> SQANLMRLKSDLFNRSPMYPGPTKDDPLTVTLGFTLQDIVKVDSSTNEVDLVYYEQQRW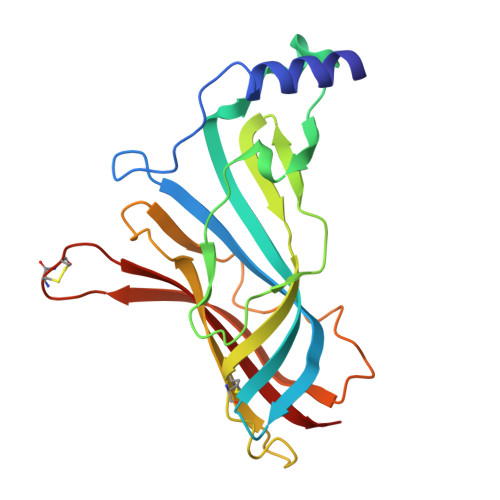KLNSLMWDPNEYGNITDFRTSAADIWTPDITAYSSTRPVQVLSPQIAVVTHDGSVMFIPAQRLSFMCDPTGVDSEEGVTCAVKFGSWVYSGFEIDLKTDTDQVDLSSYYASSKYEILSATQTRQVQHYSCCPEPYIDVNLVVKFRER> GGUUAUUCAGAUUAGGUA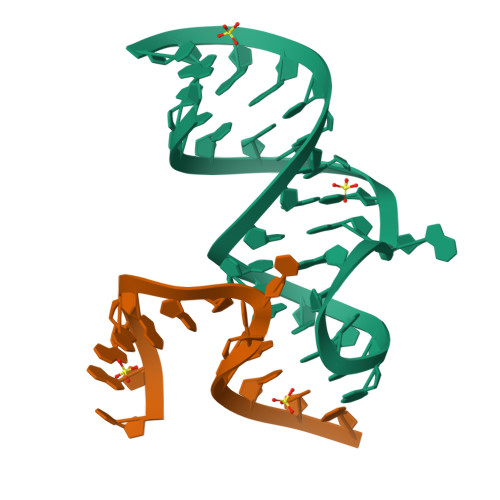GUCGAAUGACC;> UAAGAAAUUUACCU>[4x]MEALKIALLGGGTVGSAFYNLVLERAEELSAFGVVPRFLGVLVRDPRKPRAIPQELLRAEPFDLLEADLVVEAMGGVEAPLRLVLPALEA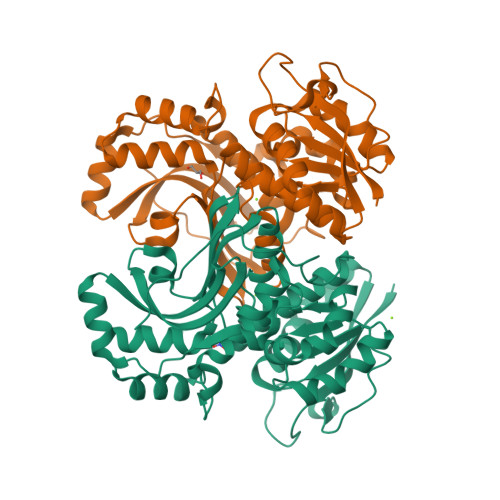GIPLITANKALLAEAWESLRPFAEEGLIYHEASVMAGTPALSFLETLRGSELLELHGILNGTTLYILQEMEKGRTYAEALLEAQRLGYAEADPTLDVEGIDAAHKLTLLARLLVDPGFPFAEVEAQGIARLTPEVLQKAEARGERVRLVASLFGEGGRWRAAVAPRRLPQDHPLARARGNALWVRARPLGEAFVTGPGAGGGATASGLFADLLRFLSGAPGHLPAPRARPPLEEGSPWPGVE> GHMPLLSASIVSAPVVTSETYVDIPGLYLDVAKAGIRDGKLQVILNVPTPYATGNNFPGIYFAIATNQGVVADGCFTYSSKVPESTGRMPFTLVATIDVGSGVTFVKGQWKSVRGSAMHIDSYA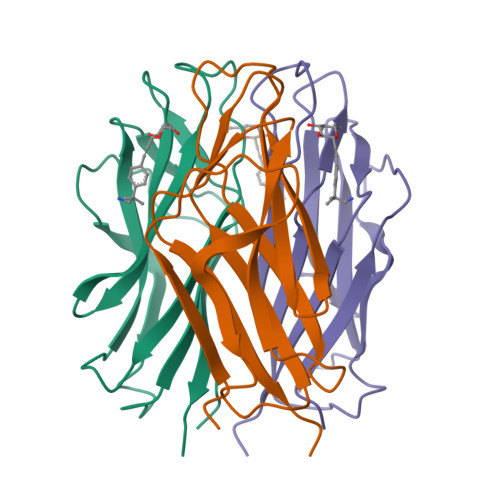SLSAIWGTAA CYCLOPROPYL-{4-[5-(3,4-DICHLOROPHENYL)-2-[(1-METHYL)-PIPERIDIN]-4-YL-3-PROPYL-3H-IMIDAZOL-4-YL]-PYRIMIDIN-2-YL}AMINE 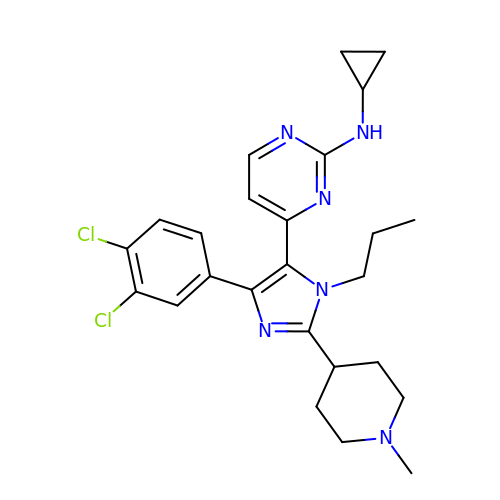| C25 H30 Cl2 N6 | XCTKFTOEAKJMII-UHFFFAOYSA-N>[4x]MEAPAAVVTGAAKRIGRAIAVKLHQTGYRVVIHYHNSAEAAVSLADELNKERSNTAVVCQADLTNSNVLPASCEEIINSCFRAFGRCDVLVNNASAFYPTPLVQGDHEDNSNGKTVETQVAELIGTNAIAPFLLTMSFAQRQKGTNPNCTSSNLSIVNLCDAMVDQPCMAFSLYNMGKHALVGLTQSAALELAPYGIRVNGVAPGVSLLPVAMGEEEKDKWRRKVPLGRREASAE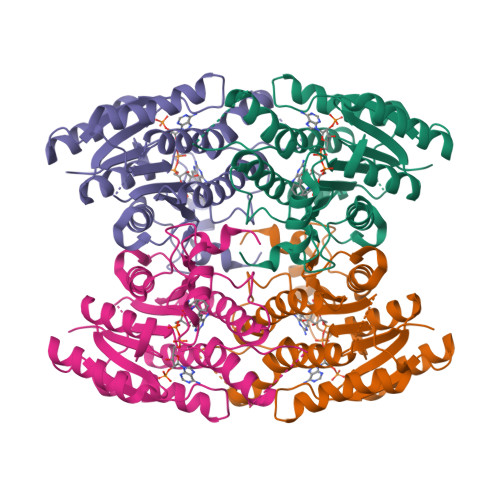QIADAVIFLVSGSAQYITGSIIKVDGGLSLVHA(2~{R})-2-[[(1~{S})-1-[(6~{S})-2-azanyl-1,4,5,6-tetrahydropyrimidin-6-yl]-2-[[(2~{S})-3-methyl-1-oxidanylidene-1-[[(2~{S})-1-oxidanyl-3-phenyl-propan-2-yl]amino]butan-2-yl]amino]-2-oxidanylidene-ethyl]carbamoylamino]-3-(4-hydroxyphenyl)propanoic 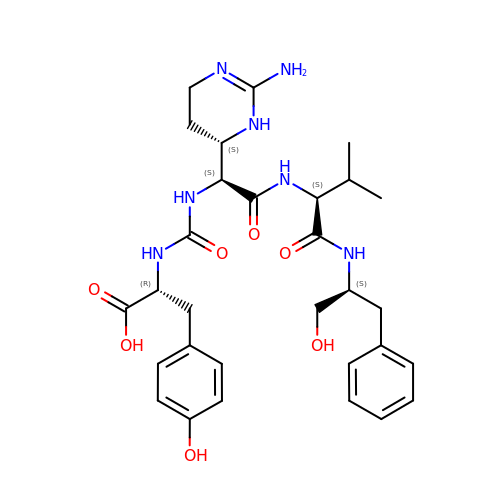acid | C30 H41 N7 O7 | JRKYEAYRXQTOFS-JRBASJLZSA-N In the mevalonate pathway, the mevalonate diphosphate decarboxylase (MDD, EC: 4.1.1.33) is a rate-limiting enzyme, suggesting that inhibition of MDD could eliminate the products of the mevalonate pathway and accordingly shut down bacterial growth. The γ-phosphate group of ATP is transferred to MVAPP to make the 3′-phosphate-MVAPP intermediate, which is then subjected to dephosphorylation and decarboxylation to produce IPP. In this study, we utilized MDD from Enterococcus faecalis V583 (MDDEF), a VRE strain, and investigated the enzyme from structural, functional and biophysical points of view. Our present results suggest that the substrate-binding mechanism of MDDs involves programmed conformational rearrangements in and around the active site, including movements of the β10-α4 loop, the phosphate-binding loop, and three helices, α1, α2, and α4.

The investigation of the structural details of the MDDEF mechanism was aided by the discovery of crystallization conditions under which the introduction of substrates and cofactors by soaking resulted in activity in the crystal. These MDDEF crystals were grown at a high ammonium sulfate concentration (1.6 M)19 but subjected to buffer exchange into PEG3350 solutions before soaking with ligands. The apo form of MDDEF (MDDEF-SO42−) has almost identical secondary structure elements compared with other MDDs. In the present structural study, the positions of two loops were determined in the ligand-bound MDDEF structures but not in apo-MDDEF. Other MVAPP-bound MDDs have stabilized phosphate-binding loops possibly due to crystal contacts directly involving this loop or the C-terminal insertion covering the corresponding β-strands in eukaryotic MDDs. In contrast to all other published structures, in the MDDEF structures, there is no crystal contact in the regions described above, which should allow the flexible loops to take up unrestricted conformations. In the physical mechanism, the phosphate-binding loop and the β10-α4 loop may be initially dynamic or disordered in an apo structure (left).

> MHHHHHHHHGVDLGTENLYFQSNAMLSGKARAHTNIALIKYWGKANEEYILPMNSSLSLTLDAFYTETTVTFDAHYSEDVFILNGILQNEKQTKKVKEFLNLVRQQADCTWFAKVESQNFVPTAAGLASSASGLAALAGACNVALGLNLSAKDLSRLARRGSGSACRSIFGGFAQWNKGHSDETSFAENIPANNWENELAMLFILINDGEKDVSSRDGMKRTVETSSFYQGWLDNVEKDLSQVHEAIKTKDFPRLGEIIEANGLRMHGTTLGAVPPFTYWSPGSLQAMALVRQARAKGIPCYFTMDAGPNVKVLVEKKNLEALKTFLSEHFSKEQLVPAFAGPGIELFETKGMDK> PRDSYSGDAL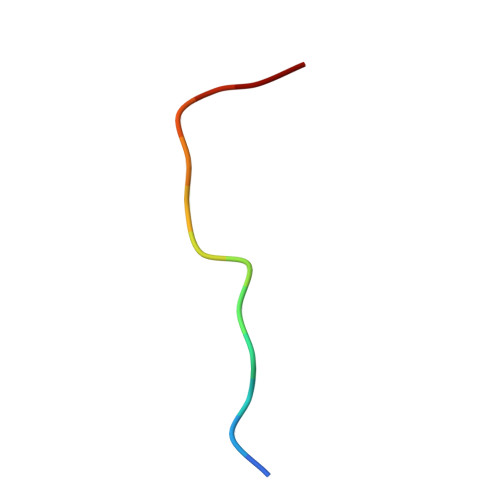YEF>[3x]MQDPIIKILIGNDTFLLGQEIIDLDFQIGEGKKQNNINFTIFDKDGFFADKYISTSYAQGGIDLPIDFLENPDDAKDTNSASTATEVDSVGNGTVSRSGVFTPKIRAFLDTIASKETAPGTALNIEGYRSVSGSSTLFDESEMVAGGFPRSQGSKNIGRYQFTVIDYNHARSKYPNINNYSPQNQDLLAYFKLQHRNVLPYLLRDDLDNAIDKASYEWASFPGIGKPQGQFNQVQSGTTIASLKSYYETRLAYYRSLEAGSDFQASAPKDTTNNQYAGKEYKTIRTLSNSTTASFYGYNDGFDSSDLTANGERFNPEGITAAHESLPFGTLVKVTWAVNNKSVVVRINDRGAFVRLGRQIDLSYGAAKALSSPGNDAIAAGLLTVKLEVVELRTPIGENLKESAKNQIAENLEKIKKNQKELATPEISAKGTQITLEVSIDRSAIAVFSFLHTGTKHNAIISDTTTFTGQSVNWVLNRRVKNTRYTGVTLKGLAATITRQYGLDLDMSEEGEMIENISQVSQTDWQFLEKMTAIQGFGMRTVGKVLQIYKITVNAKKLNYTISVVDNVKSLIVTDQAQTDATGSSQKIEHYGGRMTTVVDADSGSLIKVDKDNKREAGSAARTFTTGVDVPQPQIQKQYSNPRPEGASVKEFQLQLELHTSQSDLENLTPDTALYIENTLPFIVGKSWFIESVRHSFSEGIFTSQVSAYIPVAPKAIATDSGEQNSVVFDNSQSASQGVGKLPVYEILSYRSGRTVKKITSLQQSYEHWRGTGGYTAYKQLSGFSSPVSYMKGRPNQLVYDFILQQNGNQSCPVPSPASGRVVATGGSNGMVKIDTGGGEVRLLHMSNIRVKPGQNVIRGTILGTQASVGGTSTGTHLHIEANQFILESYVQSLVTGNW;>MIVDEFSSVYECLLYCYKMVKRSEQLNGRRVFPILSVVTNNNDPEGRRRVKIADPLFGNLIESNWIRPIRVSQNQDNPLPQINQMVIVWFVDGDSEKGYYLPIINDANPSREKDDPVNDSAVRIEGNNTIRIDKNDSETVGGNQTVAIAGEQNINVDGNLIENIGGDIDQNVTGKIEVRSESTILIDADGTIIIKNDSGAFISLGGNGEVLIQDSQGRKIRLGGAFNSTWDLNGLPMAFINATSVTIAGKQIATVGAVDTRGDTIVNKGW[3x];>[3x]MANRQHVISVDLRLLTGNFDSSLNYIQGRLNGVFGVVSDNATNSFFGNGGFLSSYLWNQAFNAIQMAGIAAFRAIGNEVKRAISYQDNLISMATSYKGLLNLTTKEAFGLARESNIIFQQRNVGLPTFGNFGTQLRAQYGDDFLSAFYDQNNMKGSLERTADMIGRTTVLLGSISGVTNYQRTSFLSNFLSDD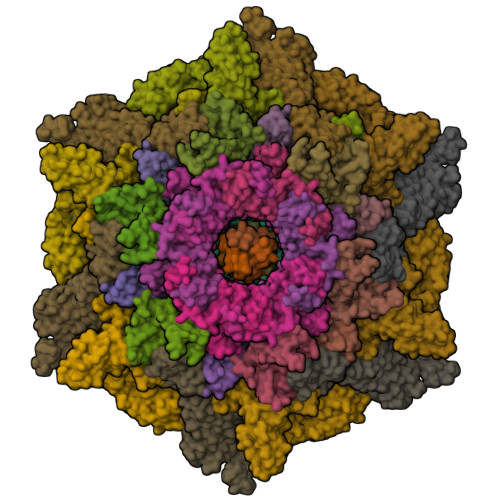FKKLQRLEVFRNSPQLQRAFNSQVDSIGGEQGFNALTRKDRLLLLENIAAIAVDDDIIKAYKDSLGGVLSRLGQELFGDIGIFSFTRDLIFGLPNTSILNSITFFMKEVFAPDGVFGLIKPALQGIVDTVLIGTKFILDRTSFIFMGLNALARVLQPIAPLIYATSSALTVLAAVGLANTIKSAVQGYLISSGAAMLGGRMGMAAMFGMGGDLVGLKTLGTLGLGKLIAPLGFLTMGLDKLADVGWLAISGGFAKAALGIKTFGMSLWAIVANPAFLTIAGIVGAIALAGYTLWKYWEPIGDFLQGFWIGFKAGLPILDQIESVLQSIGQALSPITEGFKNMASAMQPVLDGFTKFFNLQQEKGGENYVKQGVNFGDAASGVTRTILSNPLINPFSGFFGLFGNPAQNKADGDPQSVMSAINDERRKMPSGASLVIANSSENVFTRSQTQQLASAGRGSTVINNTFNISGADPQAIAKQIADIINSQWQGTLTDYA;>MTTQEFLSKNKTIESELLDLLIKPNTDDSILTRNKQAIADRDLFDIEWEPGQSLNKLATEYLGDSFAWQIIADANGIDPTKEIDIGAGLKVPDQKALENSIKKFIVNSPTGKQLISDAKQSILNLIGVGDSNTEFSKTLKDCIGKVVNFSFDNTQ[6x];>MSKFLKNRAVVNGLPVIKNPGKYQHCYLIEYEDSTNVKQTPTENKNKQQQGFPVYLFMMNPENITYNLPINYQEIAIPFTAKNQLNYSNGGNIVMTMSNLILDTMDEKRSLQPLIDRLIALREPTVKKGLKSHPKILAFKWGSNTFAPCVLTNISFDVTRWIDGYPTKARVNMSLKEIQKPSSDSKALEEAKKKVKVETVQNGNLKKTLSEKQLIDGVKRVTEYLKKNISFQPRTIQNILSDPKSVIKIDKDTGQVSLFNGNGEFAALVGTYNGDIFSPSRQ[6x];>[6x]MYVYPPRIINGTLYKSTDLAEYTRGKILQTLSIVRGELVADPFFGVPLRLFSNINDYQSDVSKIQIILEEEITEAQFIVTGDLKNNGIVSLTVYWAYLGTENIENFEIDTSNIF;>[12x]MTTDLNAPQLVVDDYEQLIIDSLVHTNVVSNGEFTDLDASGFMRPFAGTMAYAGSELLYKANLASIAAAKSFFKNVLGVPEDTGTKATTTLQFGLSASLSTDFIVPINFQVSDLSGTLRFYTIGNLVIPAGATFGTIEAIAEDIGEKYNVSANFIDQYSTPLTYLQYVTNIRPATNGRSGETIDNLIERCAQIIRIRNPVSALDFEQLAELTMGEGSRCKAIGLLGINKIVTDPQPGVVHLFLLDVNGNPADPVTISTVGATLQPRIMLGTRLLISPMEVLNIELELIALSDSSKTFQQLADDILEALKVFFNPANLTPGEPVLIEEVKFAIRSVGGLSISYLQMNDNAINIPMPNQWTIPRFSYIGFELTDSEGTVYRDNVVTVTNPEE;>[6x]MSKDAFTAWNVDRRPIYSRMPKEQVGTSYHDYIATDWLTAYWDKIFIECYDKLEDLPRQFDPLQCDEEYLDFLAPLCGWTAPYWSGDYPPESKRVLLANSYSLIWRDKGSLTVLSFVLNALFINHRIFVPGSFILGQSQVSEDTLGAAGWEFEILLPRDYAENGYEFRLTLKIASLFSPLWCKYRVRYDNL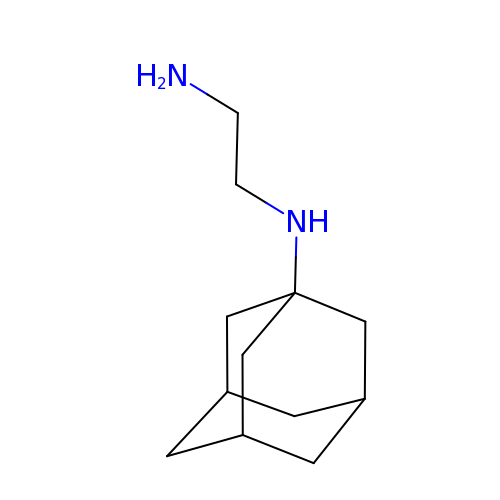N~1~-[(3s,5s,7s)-tricyclo[3.3.1.1~3,7~]decan-1-yl]ethane-1,2-diamine | C12 H22 N2 | IQMUFNISQFPZJC-CDECOKDKSA-N> GSNSHSYLSGYISLLLRAEPYPTSRFGSQCMQPNNIMGIENICELAARMLFSAVEWARNIPFFPDLQITDQVALLRLTWSELFVLNAAQCSMPLHVAPLLAAAGLHASPMSADRVVAFMDHIRIFQEQVEKLKALHVDSAEYSCLKAIVLFTSDACGLSDVAHVESLQEKSQCALEEYVRSQYPNQPTRFGKLLLRLPSLRTVSSSVIEQLFFVRLVGKTPIETLIRDMLLSGSSFNWPYMAIQ

Among the most extensively studied orphan receptors are the chicken ovalbumin upstream promoter-transcription factors (COUP-TFs), which belong to the NR2F subfamily. In mammals, the COUP-TF orphan NRs regulate many key biological processes, including angiogenesis, neuronal development, organogenesis, cell fate determination, metabolic homeostasis, and circadian rhythm. Here we demonstrate that COUP-TFII is a ligand-regulated nuclear receptor that can be activated by unphysiological micromolar concentrations of retinoic acids. COUP-TFs are the most evolutionarily conserved NRs among all species, and within the NR2F subfamily, the homology in both the DNA-binding domain (DBD) and ligand-binding domain (LBD) is extremely high.

Here we report the 1.48 Å crystal structure of the LBD of human COUP-TFII. The human COUP-TFII LBD was purified to homogeneity in a ligand-free state. There is one LBD molecule per asymmetric unit, but COUP-TFII forms a symmetric dimer through crystal packing. The structure contains 10 α helices that are folded into a typical three-layered helical sandwich seen in other NRs. The dimer interface is made up of residues involved in hydrophobic interactions and hydrogen bonding, with the majority of the hydrophobic interactions observed between residues found on the N-terminal half of helix α10 of each monomer, which forms a parallel coiled-coil structure in the crystal. In the absence of ligand, helix α10 bends at V373 and causes the C-terminal portion of α10 to collapse into the lower half of the receptor, the region where ligands have been found to bind in other NR LBDs. Due to the bulky size of these aromatic side chains and the dense pack of the binding pocket in COUP-TFII, there is no room for any ligand to bind in this conformation. The kink in helix α10 and the subsequent collapse of the binding pocket of COUP-TFII allows the AF2 helix, which follows α10, to bind in the cofactor binding site of the LBD. The N-terminal end of AF2 is stabilized by a hydrogen bond between Q393 (AF2) and R246 (α4), and the C-terminal end of the AF2 is stabilized by hydrogen bonding between the conserved charge clamp residue R228 (α3) and two backbone carbonyl groups from residues M399 and L400 (AF2). In this orientation of the AF2 helix, neither coactivators nor corepressors are able to bind to COUP-TFII, and therefore this structure represents an autorepressed form of this orphan NR.> ADNRPEKWVKGVCRYCGTGCGVLVGVKDGKAVAIQGNPNNHNAGLLCLKGSLLIPVLNSKERVTQPLVRRHKGGKLEPVSWDEALDLMASRFRSSIDMYGPNSVAWYGSGQCLTEESYVANKIFKGGFGTNNVDGNPRLCMASAVGGYVTSFGKDEPMGTYADIDQATCFFIIGSNTSEAHPVLFRRIARRKQVEPGVKIIVADPRRTNTSRIADMHVAFRPGTDLAFMHSMAWVIINEELDNPRFWQRYVNFMDAEGKPSDFEGYKAFLENYRPEKVAEICRVPVEQIYGAARAFAESAATMSLWCMGINQRVQGVFANNLIHNLHLITGQICRPGATSFSLTGQPNACGGVRDGGALSHLLPAGRAIPNAKHRAEMEKLWGLPEGRIAPEPGYHTVALFEALGRGDVKCMIICETNPAHTLPNLNKVHKAMSHPESFIVCIEAFPDAVTLEYADLVLPPAFWCERDGVYGCGERRYSLTEKAVDPPGQCRPTVNTLVEFARRAGVDPQLVNFRNAEDVWNEWRMVSKGTTYDFWGMTRERLRKESGLIWPCPSEDHPGTSLRYVRGQDPCVPADHPDRFFFYGKPDGRAVIWMRPAKGAAEEPDAEYPLY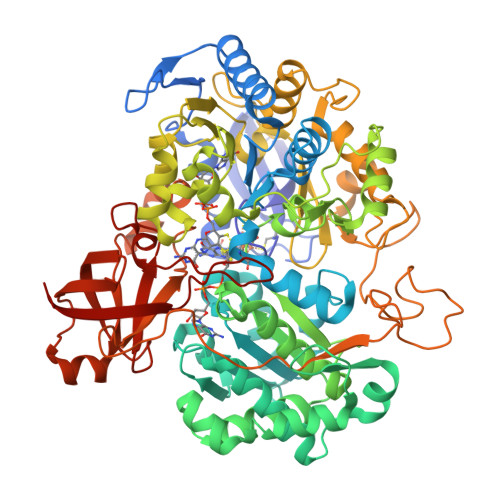LTSMRVIDHWHTATMTGKVPELQKANPIAFVEINEEDAARTGIKHGDSVIVETRRDAMELPARVSDVCRPGLIAVPFFDPKKLVNKLFLDATDPVSREPEYKICAARVRKA>[2x]SMKRGRGGRVDPFEFVTYSGEEIKESSSEERVKEGANKSSPTRTRILSAALSPAERAIFDVPIEKWLSIDRSSLS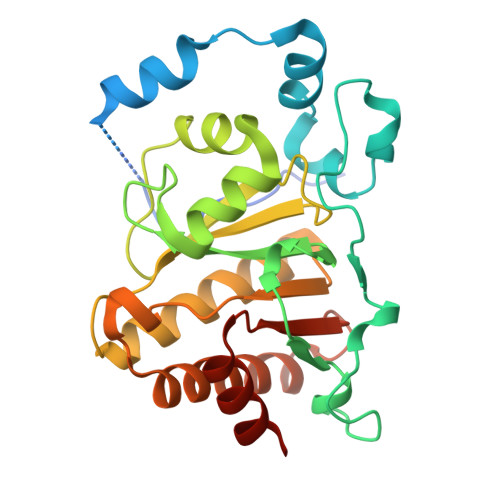GWKCAVPRPVTIEQLRPVDPSDAILRHIALYRGPVTDLQLDAIVNAANTRCLGGGGVDGAIHRVAGPLLLRECATFNGCQTGECRLTKGYQLPARYVLHTVGPVGERPDMLRKCYRSILSLALKNGLRSIGFCCVSTGVYGYPLLPATRIALGETRKFLEEHGGALDMCCFACFQEDEYKTYEKCVGKSSL> SASYKPVFVTEITDDLHFYVQDVETGTQFEKLMENMRNDIASHPPVEGSYAPRRGEFCIAKFVDGEWYRARVEKVESPAKIHVFYIDYGNREVLPSTRLGTLSPAFSTRVLPAQATEYAFAFIQVPQDDDARTDAVDSVVRDIQNTQCLLNVEHLSAGCPHVTLQFADSKGDVGLGL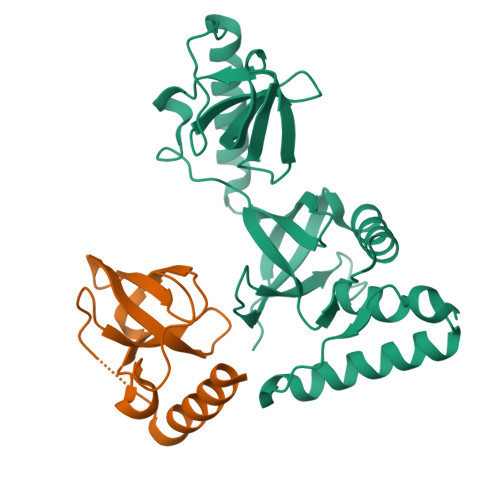VKEGLVMVEVRKEKQFQKVITEYLNAQESAKSARLNLWRY;> TQFEKLMENMRNDIASHPPVEGSYAPRRGEFCIAKFVDGEWYRARVEKVESPAKIHVFYIDYGNREVLPSTRLGTLSPAFSTRVLPAQATE> QLQRLEKSIRNNFLFNKLDSDSKRLVINCLEEKSVPKGATIIKQGDQGDYFYVVEKGTV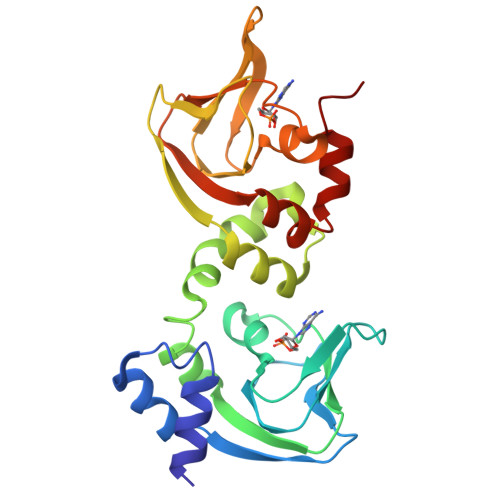DFYVNDNKVNSSGPGSSFGELALMYNSPRAATVVATSDCLLWALDRLTFRKILLGSSFKKRLMYDDLLKSMPVLKSLTTYDRAKLADALDTKIYQPGETIIREGDQGENFYLIEYGAVDVSKKGQGVINKLKDHDYFGEVALLNDLPRQATVTATKRTKVATLGKSGFQRLLGPAVDVLKLNDPTRH> MEIPVIEPLFTKVTEDIPGAMGPVFDKNGDFYIVAPSVEVNGKPAGEILRIDLKTGKKTVICKPEVNGYGGIPAGCQCDRDANQLFVADMRLGLLVVQTDGTFEEIAKKDSEGRRMQGCAYCAFDYEGNLWITAPAGEVAPADFTISLQEKFGSIYCFTTDGQMIQVDTAFQXPAGIAVRHMNDGRPYQLIVAEQPTKK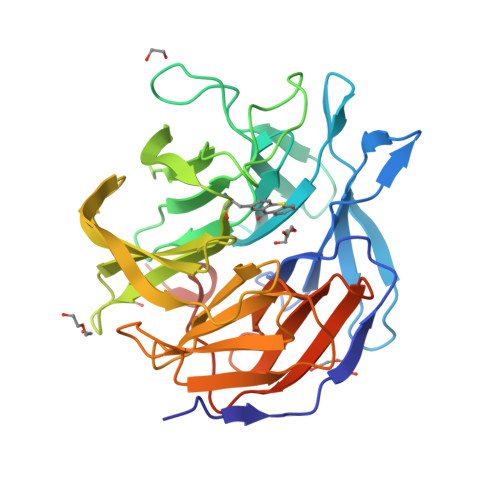LWSYDIKGPAKIENKKVWGHIPGTHEGGAAGMDFDEDNNLLVANRGSSHIEVFGPKGGQPKMRIRCPFEKPSALHFKPQTKTIFVTEHENNAVWKFEWQRNGKKQYCETLKFGIFGSLEWSHPQFEK> MSSIINKEVQEAPLKWVKNWSDEEIKALVDEEKGLLDPRIFSDQDLYEIELERVFARSWLLLGHEGHIPKAGDYLTTYMGEDPVIVVRQKDRSIKVFLNQCRHRGMRIERSDFGNAKSFTCTYHGWAYDTAGNLVNVPYEKEAFCDKKEGDCGFDKADWGPLQARVDTYKGLIFANWDTEAPDLKTYLSDATPYMDVMLDRTEAVTQVITGMQKTVIPCNWKFAAEQFCSDMYHAGTMAHLSGVLSSLPPEMDLSQVKLPSSGNQFRAKWGGHGTGWFNDDFALLQAIMGPKVVDYWTKGPAAERAKERLGKVLPADRMVAQHMTIFPTCSFLPGINTVRT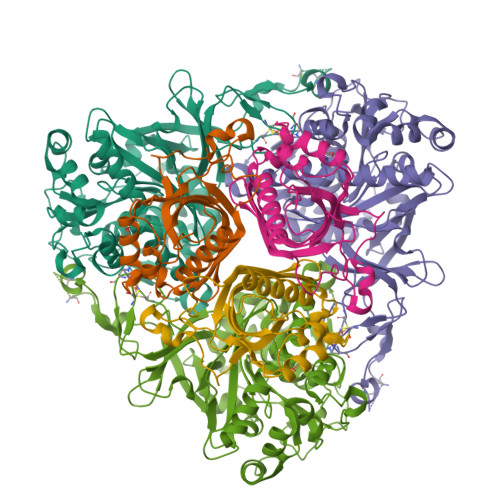WHPRGPNEIEVWSFIVVDADAPEDIKEEYRRKNIFTFNQGGTYEQDDGENWVEVQRGLRGYKARSRPLCAQMGAGVPNKNNPEFPGKTSYVYSEEAARGFYHHWSRMMSEPSWDTLKS;> MTSADLTKPIEWPEMPVSLELQNAVEQFYYREAQLLDYQNYEAWLALLTQDIQYWMPIRTTHTSRNKAMEYVPPGGNAHFDETYESMRARIRARVSGLNWTEDPPSRSRHIVSNVIVRETESAGTLEVSSAFLCYRNRLERMTDIYVGERRDILLRVSDGLGFKIAKRTILLDQSTITANNLSQFF> ALLEKVDPNKIYTIDEAAHLVKELATAKFDETVEVHAKLGIDPRRSDQNVRGTVSLPHGLGKQVRVLAIAKGEKIKEAEEAGADYVGGEEIIQKILDGWMDFDAVVATPDVMGAVGSKLGRILGPRGLLPNPKAGTVGFNIGEIIREIKAG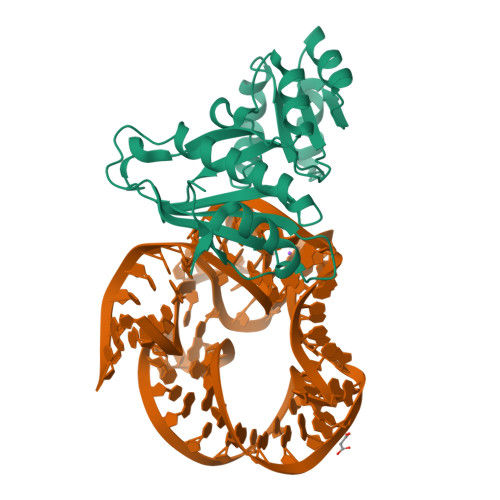RIEFRNDKTGAIHAPVGKASFPPEKLADNIRAFIRALEAHKPEGAKGTFLRSVYVTTTMGPSVRINPHS Escherichia coli phage SU10 belongs to the genus Kuravirus from the class Caudoviricetes of phages with short non-contractile tails. Here we show that the virion of SU10 has a prolate head, containing genome and ejection proteins, and a tail, which is formed of portal, adaptor, nozzle, and tail needle proteins and decorated with long and short fibers. In contrast to other short-tailed phages, the tails of Kuraviruses elongate upon cell attachment. After binding to the host, SU10 tail, nozzle proteins, and short fibers re-arrange to form a nozzle that extends the tail.

The capsid is closed on both ends with caps formed by the major capsid proteins organized with local T = 4 quasi-icosahedral symmetry. The portal complex of SU10 is embedded in the capsid at one of its fivefold vertices, where it replaces a pentamer of capsid proteins. All hexamer-hexamer and hexamer-pentamer interfaces in the caps are arched (145°), however, the hexamers that form the tubular part of the capsid are connected by two types of interfaces, arched (145°) and more planar (160°).

>MANPTLFVSYDQNGKKLSFANWISVLSPQDTPFVSMTGKESINQTIFSWQTDALASVDGNNAHVEGSRAEDGEMKPTVIKSNVTQILRKVVRVSDTANTTANYGRGRELMYQLEKKGKEIKRDLEKILLSGQARTDVLADQYLTNSAADPAVAGLNDTHAARKTGAFQFLCAHGGLAGGVVDKTKNGPADPDTGAVTVKVAQNASNPTTNIGFDEADIFDMTLQLYTAGSEADIIMINPAHAKIFAGLQENTQGSRKRIFENTKQFIYEVNSITDPLGQSYKIIVNRWMPTDAVYFFRSADWTQMVLRAPKRTELAKDGSYEKWMIEMEVGLRHRNPYASGVLFTAAGKAAA[17x]>[2x]MSTRKAVIGYYFIP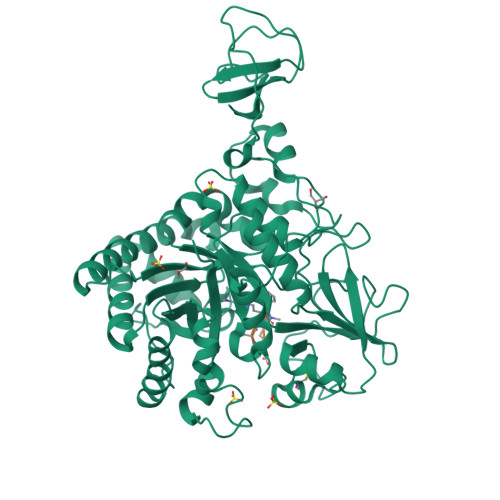TNQINNYTETDTSVVPFPVSNITPAKAKQLTHINFSFLDINSNLECAWDPATNDAKARDVVNRLTALKAHNPSLRIMFSIGGWYYSNDLGVSHANYVNAVKTPASRTKFAQSCVRIMKDYGFDGVDIDWEYPQAAEVDGFIAALQEIRTLLNQQTITDGRQALPYQLTIAGAGGAFFLSRYYSKLAQIVAPLDYINLMTYDLAGPWEKVTNHQAALFGDAAGPTFYNALREANLGWSWEELTRAFPSPFSLTVDAAVQQHLMMEGVPSAKIVMGVPFYGRAFKGVSGGNGGQYSSHSTPGEDPYPSTDYWLVGCEECVRDKDPRIASYRQLEQMLQGNYGYQRLWNDKTKTPYLYHAQNGLFVTYDDAESFKYKAKYIKQQQLGGVMFWHLGQDNRNGDLLAALDRYFNAADYDDSQLDMGTGLRYTGVGPGNLPIMTAPAYVPGTTYAQGALVSYQGYVWQTKWGYITSAPGSDSAWLKVGRVA;>XFDDA[2x]> MSLAIDLEVKQDVLIVRLSGELDHHTAEELREQVTDVLENRAI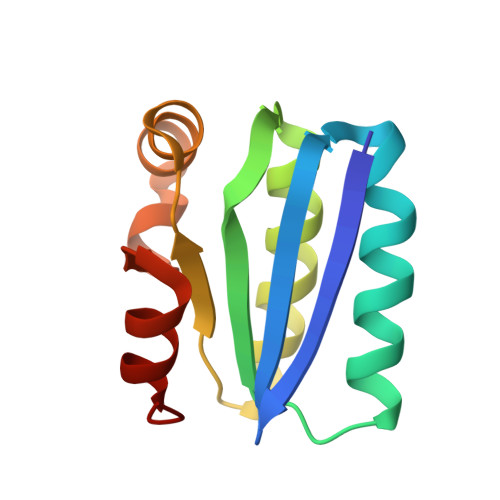RHIVLNLGQLTFMDSSGLGVILGRYKQIKNVGGQMVVCAVSPAVKRLFDMSGLFKIIRVEADEQFALQALGVA> MLRNGSLRQSLRTLDSFSLAPEDVLKTAIKTVEDYEGDNIDSNGEIKITRDAKEEVVNKVSIPQLYRYTTTLEKLLLFIGTLVAVITGAGLPLMSILQGKVSQAFINEQIVINNNGSTFLPTGQNYTKTDFEHDVMNVVWSYAAMTVGMWAAGQITVTCYLYVAEQMNNRLRREFVKSILRQEISWFDTNHSGTLATKLFDNLERVKEGTGDKIGMAFQYLSQFITGFIVAFTHSWQLTLVMLAVTPIQALCGFAIAKSMSTFAIRETLRYAKAGKVVEETISSIRTVVSLNGLRYELERYSTAVEEAKKAGVLKGLFLGISFGAMQASNFISFALAFYIGVGWVHDGSLNFGDMLTTFSSVMMGSMALGLAGPQLAVLGTAQGAASGIYEVLDRKPVIDSSSKAGRKDMKIKGDITVENVHFTYPSRPDVPILRGMNLRVNAGQTVALVGSSGCGKSTIISLLLRYYDVLKGK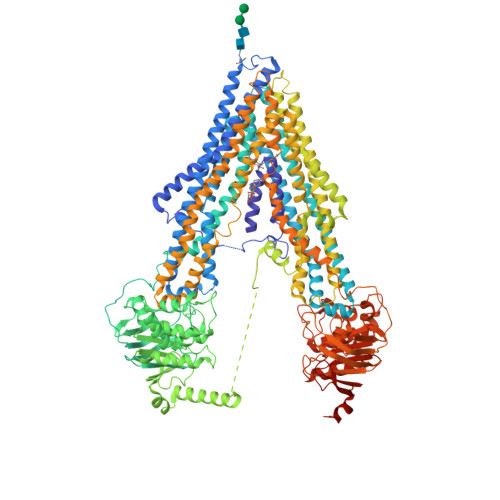ITIDGVDVRDINLEFLRKNVAVVSQEPALFNCTIEENISLGKEGITREEMVAACKMANAEKFIKTLPNGYNTLVGDRGTQLSGGQKQRIAIARALVRNPKILLLDEATSALDAESEGIVQQALDKAAKGRTTIIIAHRLSTIRNADLIISCKNGQVVEVGDHRALMAQQGLYYDLVTAQTFTDAVDSAAEGKFSRENSVARQTSEHEGLSRQASEMDDIMNRVRSSTIGSITNGPVIDEKEERIGKDALSRLKQELEENNAQKTNLFEILYHARPHALSLFIGMSTATIGGFIYPTYSVFFTSFMNVFAGNPADFLSQGHFWALMFLVLAAAQGICSFLMTFFMGIASESLTRDLRNKLFRNVLSQHIGFFDSPQNASGKISTRLATDVPNLRTAIDFRFSTVITTLVSMVAGIGLAFFYGWQMALLIIAILPIVAFGQYLRGRRFTGKNVKSASEFADSGKIAIEAIENVRTVQALAREDTFYENFCEKLDIPHKEAIKEAFIQGLSYGCASSVLYLLNTCAYRMGLALIITDPPTMQPMRVLRVMYAITISTSTLGFATSYFPEYAKATFAGGIIFGMLRKISKIDSLSLAGEKKKLYGKVIFKNVRFAYPERPEIEILKGLSFSVEPGQTLALVGPSGCGKSTVVALLERFYDTLGGEIFIDGSEIKTLNPEHTRSQIAIVSQEPTLFDCSIAENIIYGLDPSSVTMAQVEEAARLANIHNFIAELPEGFETRVGDRGTQLSGGQKQRIAIARALVRNPKILLLDEATSALDTESEKVVQEALDRAREGRTCIVIAHRLNTVMNADCIAVVSNGTIIEKGTHTQLMSEKGAYYKLTQKQMTEKK methyl 4'-(alpha-D-mannopyranosyloxy)biphenyl-3-carboxylate 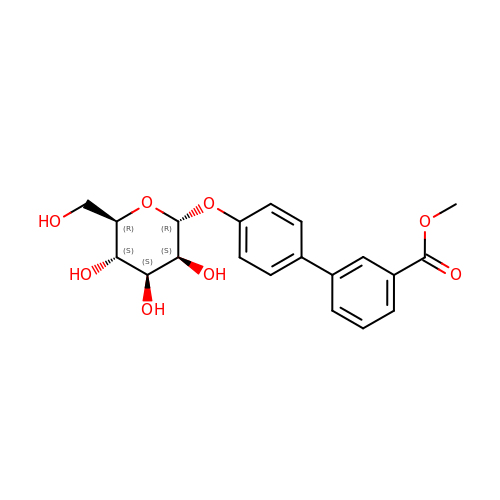| C20 H22 O8 | GDSLRMGPZWIAEZ-JGLNRKDHSA-N> MHHHHHHMNFNVSLMEKLKWKIKCIENKFLNYRLTTNETVVAETEYGKVKGVKRLTVYDDSYYSFEGIPYAQPPVGELRFKAPQRPTPWAGVRDCCNHKDKSVQVDFITGKVCGSEDCLYLSVYTNNLNPETKRPVLVYIHGGGFIIGENHRDMYGPDYFIKKDVVLINIQYRLGALGFLSLNSEDLNVPGNAGLKDQVMALRWIKNNCANFGGNPDNITVFGESAGAASTHYMMLTEQTRGLFHRGILMSGNAICPWANTQCQHRAFTLAKLAGYKGEDN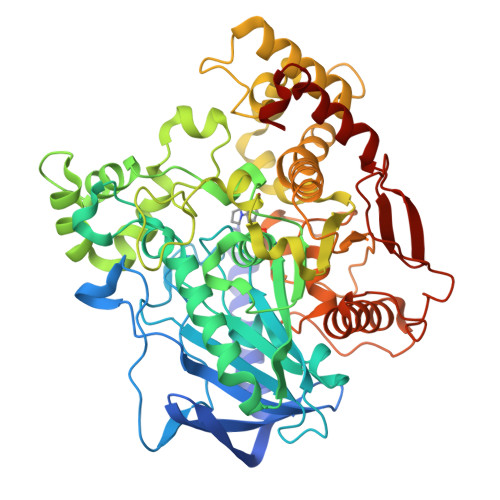DKDVLEFLMKAKPQDLIKLEEKVLTLEERTNKVMFPFGPTVEPYQTADCVLPKHPREMVKTAWGNSIPTMMGNTSYEGLFFTSILKQMPMLVKELETCVNFVPSELADAERTAPETLEMGAKIKKAHVTGETPTADNFMDLCSHIYFWFPMHRLLQLRFNHTSGTPVYLYRFDFDSEDLINPYRIMRSGRGVKGVSHADELTYFFWNQLAKRMPKESREYKTIERMTGIWIQFATTGNPYSNEIEGMENVSWDPIEKSDEVYKCLNISDELKMIDVPEMDKIKQWESMFEKHRDLF(2-fluoranyl-4-methoxy-phenyl)-[(3~{R},5~{R})-4-(2-fluoranyl-4-methoxy-phenyl)carbonyl-3,5-dimethyl-piperazin-1-yl]methanone 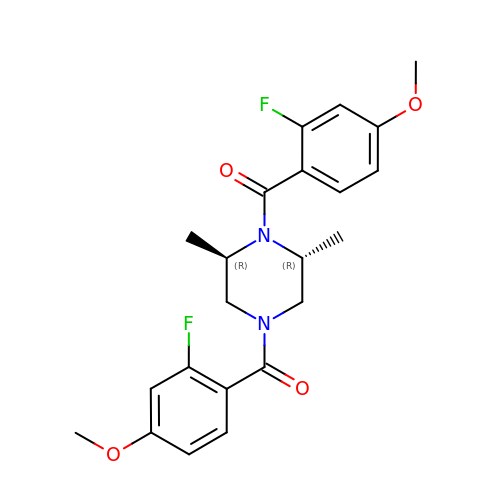| C22 H24 F2 N2 O4 | AXEACVXVOQJBDU-ZIAGYGMSSA-N>[2x]AMNAYYIQDRLEAQSWARHYQQLAREEKEAELADDMEKGIPQHLFESL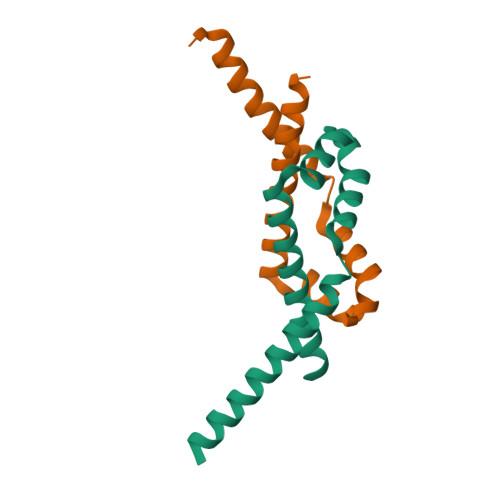CIDHLQRHGASKKSITRAFDDDVEFQERMAEHIRYMVETIAHHQVDIDSEV>[2x]MALVLEIFTLLASICWVSANIFEYQVDAQPLRPCELQRETAFLKQADYVPQCAEDGSFQTVQCQNDGRSCWCVGANGSEVLGSRQPGRPVACLSFCQLQKQQILLSGYINSTDTSYLPQCQDSGDYAPVQC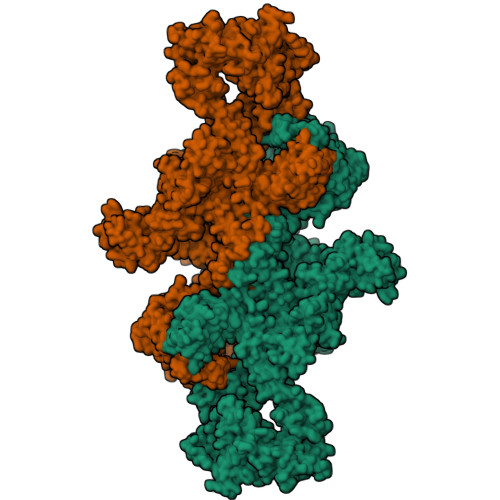DVQQVQCWCVDAEGMEVYGTRQLGRPKRCPRSCEIRNRRLLHGVGDKSPPQCSAEGEFMPVQCKFVNTTDMMIFDLVHSYNRFPDAFVTFSSFQRRFPEVSGYCHCADSQGRELAETGLELLLDEIYDTIFAGLDLPSTFTETTLYRILQRRFLAVQSVISGRFRCPTKCEVERFTATSFGHPYVPSCRRNGDYQAVQCQTEGPCWCVDAQGKEMHGTRQQGEPPSCAEGQSCASERQQALSRLYFGTSGYFSQHDLFSSPEKRWASPRVARFATSCPPTIKELFVDSGLLRPMVEGQSQQFSVSENLLKEAIRAIFPSRGLARLALQFTTNPKRLQQNLFGGKFLVNVGQFNLSGALGTRGTFNFSQFFQQLGLASFLNGGRQEDLAKPLSVGLDSNSSTGTPEAAKKDGTMNKPTVGSFGFEINLQENQNALKFLASLLELPEFLLFLQHAISVPEDVARDLGDVMETVLSSQTCEQTPERLFVPSCTTEGSYEDVQCFSGECWCVNSWGKELPGSRVRGGQPRCPTDCEKQRARMQSLMGSQPAGSTLFVPACTSEGHFLPVQCFNSECYCVDAEGQAIPGTRSAIGKPKKCPTPCQLQSEQAFLRTVQALLSNSSMLPTLSDTYIPQCSTDGQWRQVQCNGPPEQVFELYQRWEAQNKGQDLTPAKLLVKIMSYREAASGNFSLFIQSLYEAGQQDVFPVLSQYPSLQDVPLAALEGKRPQPRENILLEPYLFWQILNGQLSQYPGSYSDFSTPLAHFDLRNCWCVDEAGQELEGMRSEPSKLPTCPGSCEEAKLRVLQFIRETEEIVSASNSSRFPLGESFLVAKGIRLRNEDLGLPPLFPPREAFAEQFLRGSDYAIRLAAQSTLSFYQRRRFSPDDSAGASALLRSGPYMPQCDAFGSWEPVQCHAGTGHCWCVDEKGGFIPGSLTARSLQIPQCPTTCEKSRTSGLLSSWKQARSQENPSPKDLFVPACLETGEYARLQASGAGTWCVDPASGEELRPGSSSSAQCPSLCNVLKSGVLSRRVSPGYVPACRAEDGGFSPVQCDQAQGSCWCVMDSGEEVPGTRVTGGQPACESPRCPLPFNASEVVGGTILCETISGPTGSAMQQCQLLCRQGSWSVFPPGPLICSLESGRWESQLPQPRACQRPQLWQTIQTQGHFQLQLPPGKMCSADYADLLQTFQVFILDELTARGFCQIQVKTFGTLVSIPVCNNSSVQVGCLTRERLGVNVTWKSRLEDIPVASLPDLHDIERALVGKDLLGRFTDLIQSGSFQLHLDSKTFPAETIRFLQGDHFGTSPRTWFGCSEGFYQVLTSEASQDGLGCVKCPEGSYSQDEECIPCPVGFYQEQAGSLACVPCPVGRTTISAGAFSQTHCVTDCQRNEAGLQCDQNGQYRASQKDRGSGKAFCVDGEGRRLPWWETEAPLEDSQCLMMQKFEKVPESKVIFDANAPVAVRSKVPDSEFPVMQCLTDCTEDEACSFFTVSTTEPEISCDFYAWTSDNVACMTSDQKRDALGNSKATSFGSLRCQVKVRSHGQDSPAVYLKKGQGSTTTLQKRFEPTGFQNMLSGLYNPIVFSASGANLTDAHLFCLLACDRDLCCDGFVLTQVQGGAIICGLLSSPSVLLCNVKDWMDPSEAWANATCPGVTYDQESHQVILRLGDQEFIKSLTPLEGTQDTFTNFQQVYLWKDSDMGSRPESMGCRKDTVPRPASPTEAGLTTELFSPVDLNQVIVNGNQSLSSQKHWLFKHLFSAQQANLWCLSRCVQEHSFCQLAEITESASLYFTCTLYPEAQVCDDIMESNAQGCRLILPQMPKALFRKKVILEDKVKNFYTRLPFQKLMGISIRNKVPMSEKSISNGFFECERRCDADPCCTGFGFLNVSQLKGGEVTCLTLNSLGIQMCSEENGGAWRILDCGSPDIEVHTYPFGWYQKPIAQNNAPSFCPLVVLPSLTEKVSLDSWQSLALSSVVVDPSIRHFDVAHVSTAATSNFSAVRDLCLSECSQHEACLITTLQTQPGAVRCMFYADTQSCTHSLQGQNCRLLLREEATHIYRKPGISLLSYEASVPSVPISTHGRLLGRSQAIQVGTSWKQVDQFLGVPYAAPPLAERRFQAPEPLNWTGSWDASKPRASCWQPGTRTSTSPGVSEDCLYLNVFIPQNVAPNASVLVFFHNTMDREESEGWPAIDGSFLAAVGNLIVVTASYRVGVFGFLSSGSGEVSGNWGLLDQVAALTWVQTHIRGFGGDPRRVSLAADRGGADVASIHLLTARATNSQLFRRAVLMGGSALSPAAVISHERAQQQAIALAKEVSCPMSSSQEVVSCLRQKPANVLNDAQTKLLAVSGPFHYWGPVIDGHFLREPPARALKRSLWVEVDLLIGSSQDDGLINRAKAVKQFEESRGRTSSKTAFYQALQNSLGGEDSDARVEAAATWYYSLEHSTDDYASFSRALENATRDYFIICPIIDMASAWAKRARGNVFMYHAPENYGHGSLELLADVQFALGLPFYPAYEGQFSLEEKSLSLKIMQYFSHFIRSGNPNYPYEFSRKVPTFATPWPDFVPRAGGENYKEFSELLPNRQGLKKADCSFWSKYISSLKTSADGAKGGQSAESEEEELTAGSGLREDLLSLQEPGSKTYSK>MAVTNEEIKTASKIVRRVSNVEAFDKSGSVFKGYQIWTDISPTIENDPNIMFVKCVVQQGSKKEKLTVVQIDPPGTGTPYDIDPTHAWNCNSQVDPMSFGDIGLLNHTNIPCVLDFLKHRYLKNQIYTTAVPLIVAINPYKDLGNTTNEWIRRYRDTADHTKLPPHVFTCAREALSNLHGVNKSQTIIVSGESGAGKTEATKQIMRYFASSKSGNMDLRIQTAIMAANPVLEAFGNAKTIRNNNSSRFGRFMQLVISHEGGIRYGSVVAFLLEKSRIITQDDNERSYHIFYQFLKGANSTMKSKFGLKGVTEYKLLNPNSTEVSGVDDVKDFEEVIESLKNMELSESDIEVIFSIVAGILTLGNVRLIEKQEAGLSDAAAIMDEDMGVFNKACELMYLDPELIKREILIKVTVAGGTKIEGRWNKNDAEVLKSSLCKAMYEKLFLWIIRHLNSRIEPEGGFKTFMGMLDIFGFEVFKNNSLEQLFINITNEMLQKNFVDIVFERESKLYKDEGISTAELKYTSNKEVINVLCEKGKSVLSYLEDQCLAPGGTDEKFVSSCATNLKENNKFTPAKVASNKNFIIQHTIGPIQYCAESFLLKNKDVLRGDLVEVIKDSPNPIVQQLFEGQVIEKGKIAKGSLIGSQFLNQLTSLMNLINSTEPHFIRCIKPNENKKPLEWCEPKILIQLHALSILEALVLRQL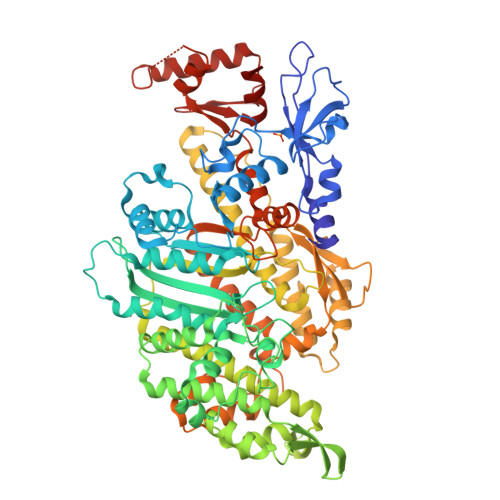GYSYRRTFEEFLYQYKFVDIAAAEDSSVENQNKCVNILKLSGLSESMYKIGKSMVFLKQEGAKILTK[4x]> MGCERKALILMVVIWIMSFWTLSLADISSTEIAVYWGQREDGLLRDTCKTNNYKI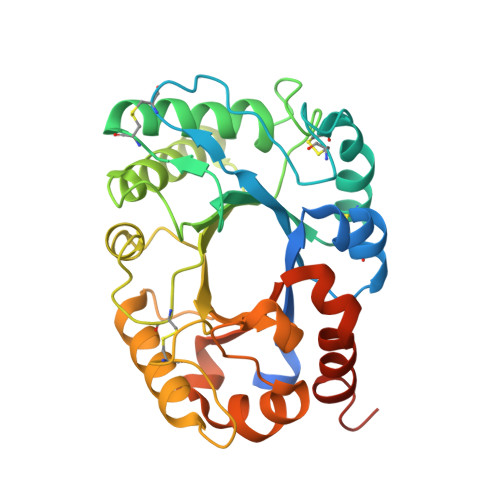VFISFLDKFGCEIRKPELELEGVCGPSVGNPCSFLESQIKECQRMGVKVFLALGGPKGTYSACSADYAKDLAEYLHTYFLSERREGPLGKVALDGIHFDIQKPVDELNWDNLLEELYQIKDVYQSTFLLSAAPGCLSPDEYLDNAIQTRHFDYIFVRFYNDRSCQYSTGNIQRIRNAWLSWTKSVYPRDKNLFLELPASQATAPGGGYIPPSALIGQVLPYLPDLQTRYAGIALWNRQADKETGYSTNIIRYLNATAMPFTSNLLKYPS>[6x]MGSTAVVHGDDLMEPTLQSILSQKTLRWIFVGGKGGVGKTTTSCSLAIQLAKVRKSVLLISTDPAHNLSDAFGQKFGKEARLVDGYSNLSAMEIDPNGSIQDLLASGDSQGDDPLAGLGMGNMMQDLAFSIPGVDEAMSFAEVLKQVKSLSYEVIVFDTAPT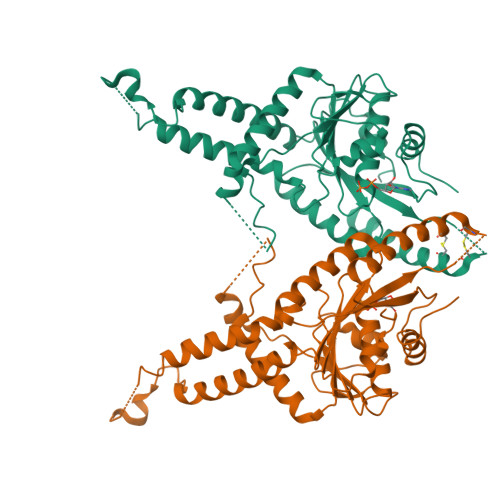GHTLRFLQFPTVLEKALAKLSQLSSQFGPMLNSILGARGGLPGGQNIDELLQKMESLRETISEVNTQFKNPDMTTFVCVCIAEFLSLYETERMIQELTSYGIDTHAIVVNQLLFPKEGSGCEQCNARRKMQKKYLEQIEELYEDFNVVRMPLLVEEVRGKEKLEKFSEMLVHPYVPPQLEHHHHHH>[8x]MEDSCVLRGVMINKDVTHPRMRRYIKNPRIVLLDSSLEYKKGESQTDIEITREEDFTRILQMEEEYIHQLCEDIIQLKPDVVI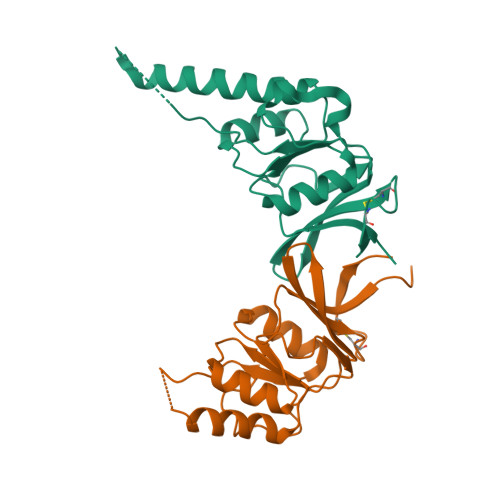TEKGISDLAQHYLMRANVTAIRRVRKTDNNRIARACGARIVSRPEELREDDVGTGAGLLEIKKIGDEYFTFITDCKDPKACTILLRGASHHHHHH> MKTTPLVHVASVEKGRSYEDFQKVYNAIALKLREDDEYDNAIGYGPVLVRLAWHTSGTWDKHD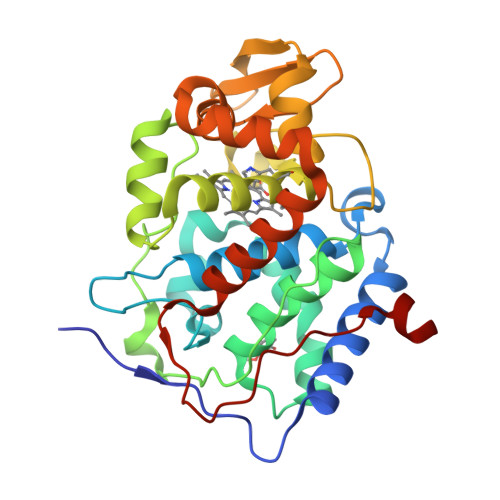NTGGSYGGTYRFKKEFNDPSNAGLQNGFKFLEPIHKEFPWISSGDLFSLGGVTAVQEWQGPKIPWRCGRVDTPEDTTPDNGRLPDADKDADYVRTFFQRLNMNDREVVALMGAHALGKTHLKNSGYEGPWGAANNVFTNEFYLNLLNEDWKLEKNDANNEQWDSKSGYMMLPTDYSLIQDPKYLSIVKEYANDQDKFFKDFSKAFEKLLENGITFPKDAPSPFIFKTLEEQGL1-[(4-methoxyphenyl)methyl]-3,4,5,6,7,8-hexahydroisoquinoline | C17 H21 N O | 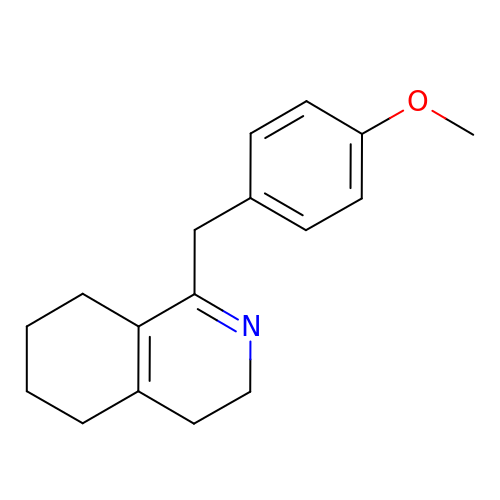IYZRINJHKVQAQC-UHFFFAOYSA-N>[8x]GSKKPRQKRTATKAYNVTQAFGRRGPEQTQGNFGDQELIRQGTDYKHWPQIAQF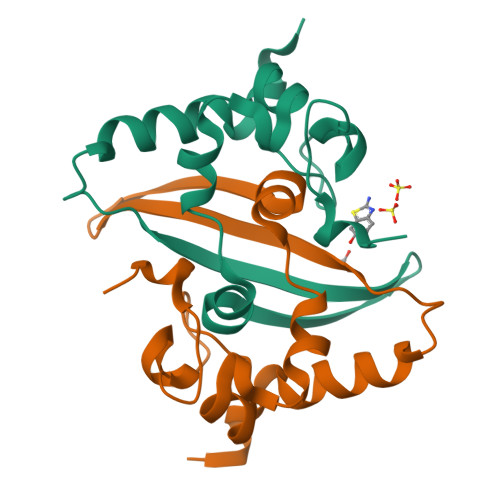APSASAFFGMSRIGMEVTPSGTWLTYTGAIKLDDKDPNFKDQVILLNKHIDAYKTFP>[2x]MNKVHVSAVGTALLKNSLSADNVKKEVEDLGLKDWDRLKFDDDRQNKIRDNFTTLKDLLLNFLKSKGKEASAELDSLLSAIEKLQHKKEELYVFLYTTNTWNSKLAGEVIKNYLEEEGIKSELAT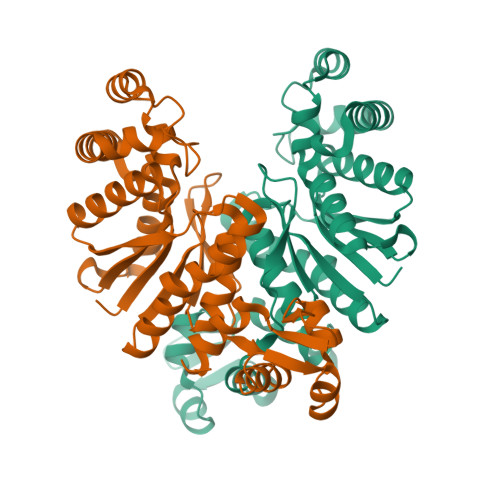VKSISSEETFHEGIEDLFDKVIYKILKFKEEGKEVYINATAGLKPETTFLTLAGLLAGADLVYYKYQEFNDVVFLPSPPITISPRYLEWLIEFANYGYTLSEKKAEELGIPVRLLEVRNLVERKGEDAYRLKDWVRKMLGIYLGSEFELE> 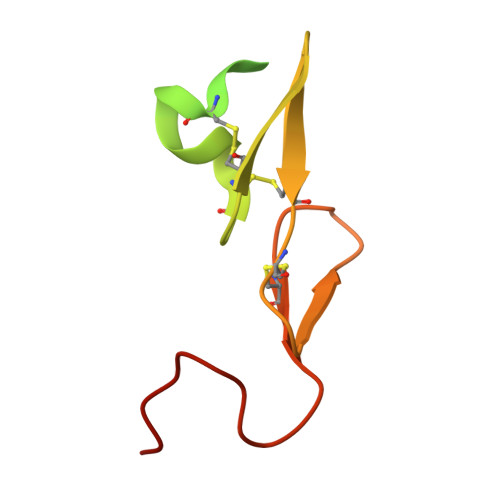YKDGDQCETSPCQNQGKCKDGLGEYTCTCLEGFEGKNCELFTRKLCSLDNGDCDQFCHEEQNSVVCSCARGYTLADNGKACIPTGPYPCGKQTLER> SMDPQTLITKANKVSYYGNPTSKESWRYDWYQPSKVSSNVQQPQQQLGDMENNLEKYP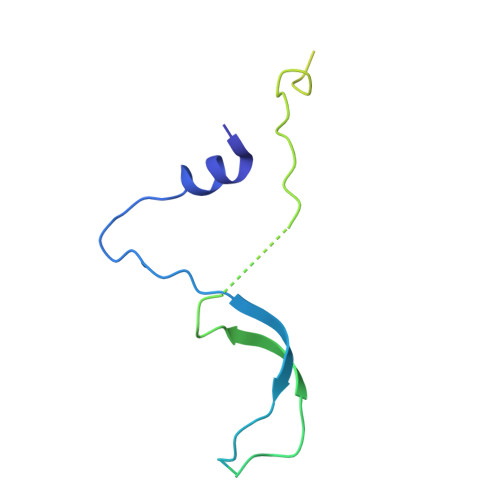FRYKTWLRNQEDEKNLQRESCEDILDLKEFDRRILKKSLMTSHTKGDTSKATGAPSANQGDEALSVDDIRGAVGNSEAIPGLSAGVNNDNTKESKDVKMN>YKDDDDKLHSQANLMRLKSDLFNRSPMYPGPTKDDPLTVTLGFTLQDIVKADSSTNEVDLVYYEQQRWKLNSLMWDPNEYGNITDFRTSAADIWTPDITAYSSTRPVQVLSPQIAVVTHDGSVMFIPAQRLSFMCDPTGVDSEEGATCAVKFGSWVYSGFEI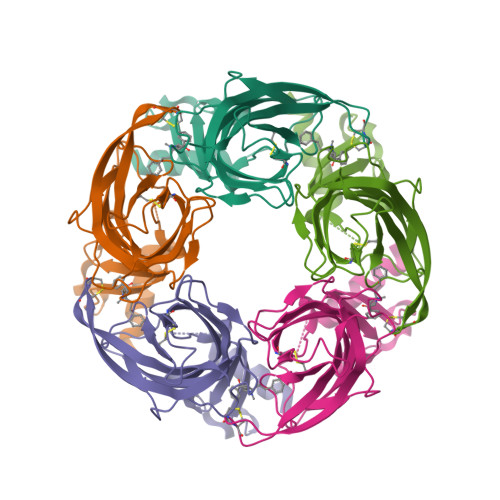DLKTDTDQVDLSSYYASSKYEILSATQTRQVQHYSCCPEPYIDVNLVVKFRERRAGNGFFRNLFD[10x]> MGKRHRNLIDQITTWENLLDAYRKTSHGKRRTWGYLEFKEYDLANLLALQAELKAGNYERGPYREFLVYEPKPRLISALEFKDRLVQHALCNIVAPIFEAGLLPYTYACRPDKGTHAGVCHVQA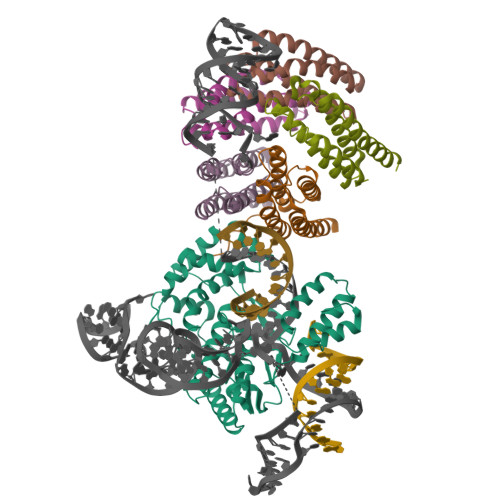ELRRTRATHFLKSDFSKFFPSIDRAALYAMIDKKIHCAATRRLLRVVLPDEGVGIPIGSLTSQLFANVYGGAVDRLLHDELKQRHWARYMDDIVVLGDDPEELRAVFYRLRDFASERLGLKISHWQVAPVSRGINFLGYRIWPTHKLLRKSSVKRAKRKVANFIKHGEDESLQRFLASWSGHAQWADTHNLFTWMEEQYGIACH;>MEPIEEATKCYDQMLIVERYERVISYLYPIAQSIPRKHGVAREMFLKCLLGQVELFIVAGKSNQVSKLYAADAGLAMLRFWLRFLAGIQKPHAMTPHQVETAQVLIAEVGRILGSWIARVNRKGTKVQVGEALVGDGNEVAHIDLIIGPRGSPAETAFCNGLVNNKHGFTSLLAVIAPNLPCKPNTLMFNKVTINDARQAVQMFGPAQHGVAMAVQDAVAEGIIPADEADDLYVLVGVFIHWEAADDAKIQKYNYEATKLSIQRAVNGEPKASVVTEQRKSATHPFAANA[5x]>[2x]SPVAGHDAVSHEEKRQSTSFWYANMDHTGNARGFAPDLDGDFSYAVYKAVAPGDAAGIQRAINEGTGGVRRHGEWLASQPRVVYIPPGTYTISSTI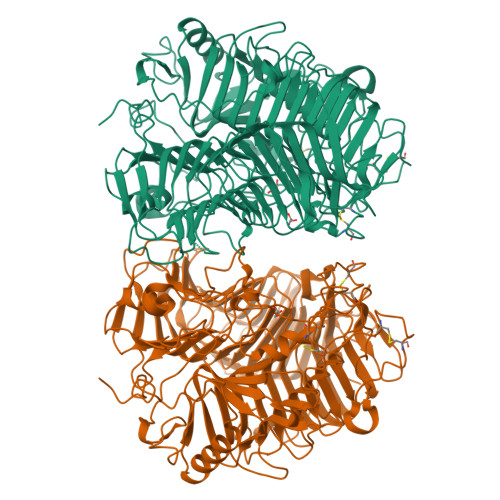FMNTDTILMGDATNPPVLKAAAGFSGNRILLDGRDPSITDGRGELSFAVGLKNLILDTTNIQGGQEFTALHWGVAQVAQLQNIKIRMSPSVSGSSTGHTGIRLTRGSTLALADVRLERGLNGIWHDGHQQALYKSIYFYQNTVGMLITNGATISILAPTFETVGTGVLCTSGAPYIGLVDARSINSGVTLKTTTYPSFLIENLNKDAQSSSNVAEGPSGTILNNRAHVDTFTYGNTVGRNPVYGDTYTTNTRPPALAPGGKYPVLPAPNYAANTVADFINVKDPAQNGGRTVLGDNTKDESKVLNEILQLAASTNKIAYFPFGKYRVDDTLLVPRGSRIVGEAWSTITGNGDKFKDESNPRPVVKVGNAGDVGVAQISDMRITISDVMPGAILIQFNMAGSNPGDVALWNSLITIGGTRGANALNSKCKDARNECKAAFLGMHFTTSSSAYVENVWNWVTDHGTEAYDSGSNIAAKGGALVESTRGTWLHALGSEHYWLYQLNLRKASNVMISLLQSETNYDQGDNVQQAPPAPWTPNVTGWGDPDFSWCGPNDTRCRMGFSNYINGGSNIYTYASASWAFFSGPGYQNCAGEFACQNHLHWIEQAPTNLQAFGICGKGSWAALRLAGGNVITSEPDFKGGWNGGGGGSLVGRYTP tert-butyl {(3S,5R)-5-[cyclopropyl(2,3-dichlorobenzyl)carbamoyl]piperidin-3-yl}carbamate | C21 H29 Cl2 N3 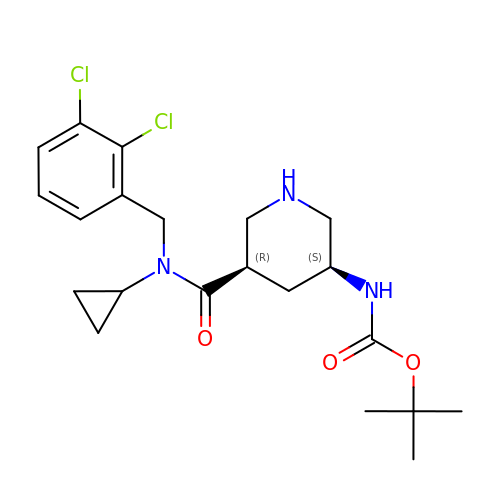O3 | VPHFZAIDKCROMZ-CABCVRRESA-N>SNAEDELYRQSLEIISRYLREQATGAKDTKPMGRSGATSRKALETLRRVGDGVQRNHETAFQGMLRKLDIKNEDDVKSLSRVMIHVFSDGVTNWGRIVTLISFGAFVAKHLKTINQESCIEPLAESITDVLVRTKRDWLVKQRGWD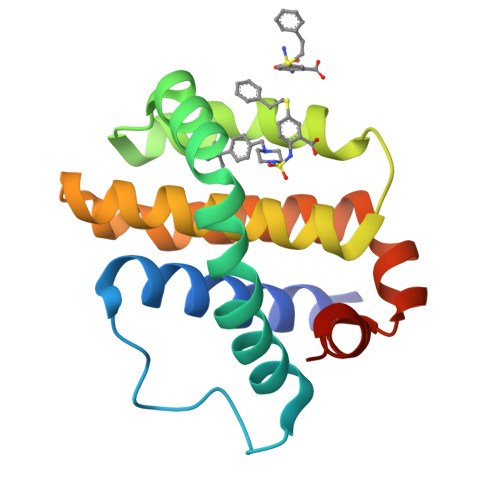GFVEFFHVED[3x]> MSQSNRELVVDFLSYKLSQKGYSWSQPMAAVKQALREAGDEFELRYRRAFSDLTSQLHITPGTAYQSFEQVVNELFRDGVNWGRIVAFF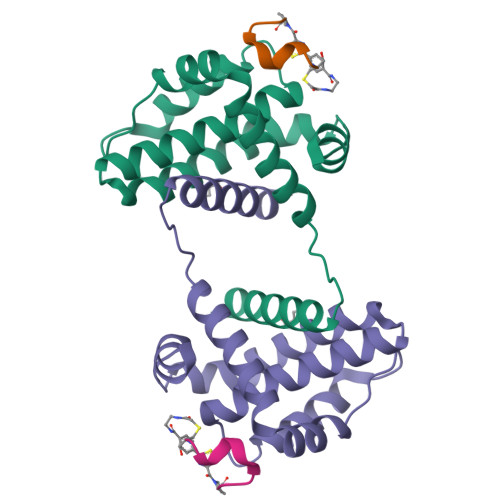SFGGALCVESVDKEMQVLVSRIASWMATYLNDHLEPWIQENGGWDTFVDLYG;> PIRYPWDVEC>[8x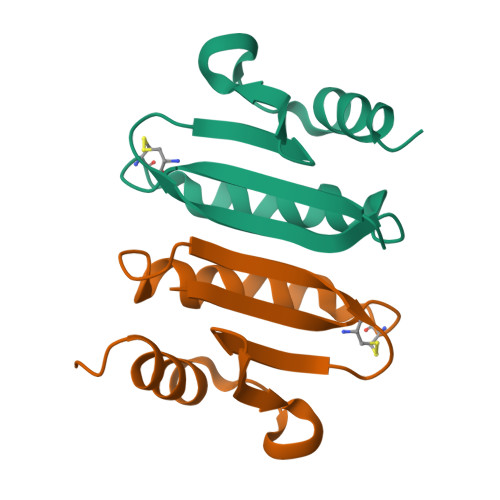]MVGAPRMTTPHTHRVQIEYCTQCRWLPRAAWLAQELLTTFETELTELALKPGTGGVFVVRVDDEVVWDRREQGFPEPTAVKRLVRDRVAPEKSLGHSERLEHHHHHH2-[3-[(4-azanyl-2-methyl-pyrimidin-5-yl)methyl]-2-[(1~{S})-1-(dioxidanyl)-1-oxidanyl-ethyl]-4-methyl-1,3-thiazol-5-yl]ethyl 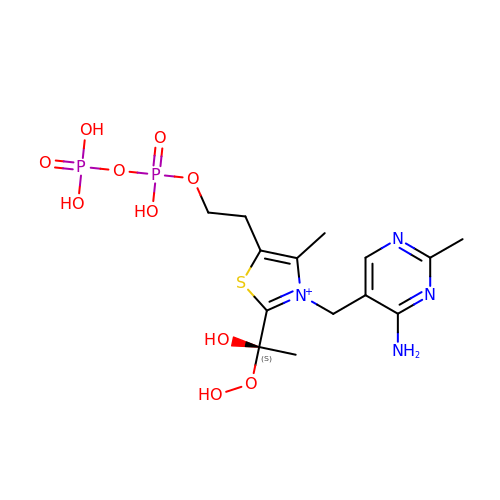phosphono hydrogen phosphate | C14 H23 N4 O10 P2 S | IMARWCCDLODQKU-AWEZNQCLSA-N> MIEKLRNIAIIAHVDHGKTTLVDKLLQQSGTFDSRAETQERVMDSNDLEKERGITILAKNTAIKWNDYRINIVDTPGHADFGGEVERVMSMVDSVLLVVDAFDGPMPQTRFVTKKAFAYGLKPIVVINKVDRPGARPDWVVDQVFDLFVNLDATDEQLDFPIVYASALNGIAGLDHEDMAEDMTPLYQAIVDHVPAPDVDLDGPFQMQISQLDYNSYVGVIGIGRIKRGKVKPNQQVTIIDSEGKTRNAKVGKVLGHLGLERIETDLAEAGDIV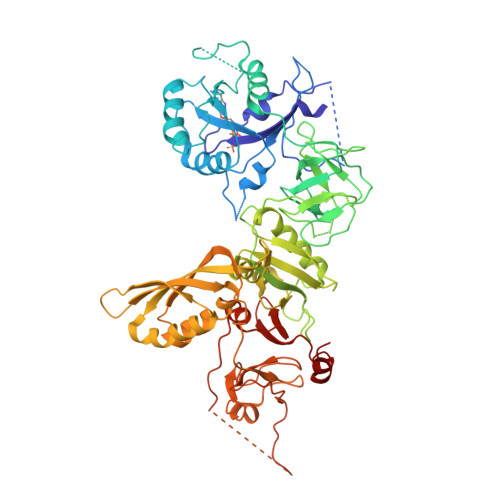AITGLGELNISDTVCDTQNVEALPALSVDEPTVSMFFCVNTSPFCGKEGKFVTSRQILDRLNKELVHNVALRVEETEDADAFRVSGRGELHLSVLIENMRREGFELAVSRPKVIFREIDGRKQEPYENVTLDVEEQHQGSVMQALGERKGDLKNMNPDGKGRVRLDYVIPSRGLIGFRSEFMTMTSGTGLLYSTFSHYDDVRPGEVGQRQNGVLISNGQGKAVAFALFGLQDRGKLFLGHGAEVYEGQIIGIHSRSNDLTVNCLTGKKLTNMRASGTDEAVVLVPPIRMTLEQALEFIDDDELVEVTPTSIRIRKRHLTENDRRRANRAPKDD>[2x]MKRVITLFAVLLMGWSVNAWSFACKTANGTAIPIGGGSANVYVNLAPVVNVGQNLVVDLSTQIFCHNDYPETITDYVTLQRGSAYGGVLSNFSGTVKYSGSSYPFPTTSETPRVVYNSRTDKPWPVALYLTPVSSAGGVAIKAGSLIAVLILRQTNNYNSDDFQFVWNIYANNDVVVPTGGCDVSARDVTVTLPDYPGSVPIPLTVYCAKSQNLGYYLSGTTADAGNSIFTNTASFSPAQGVG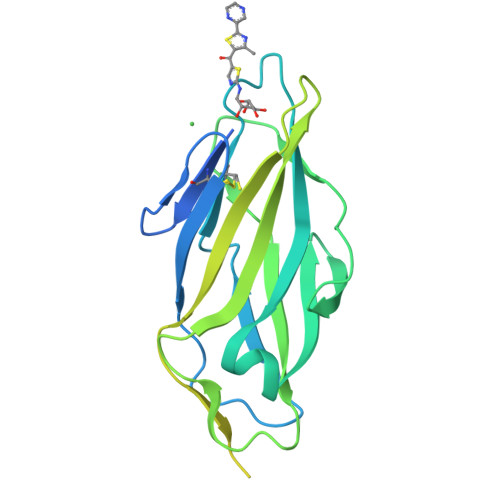VQLTRNGTIIPANNTVSLGAVGTSAVSLGLTANYARTGGQVTAGNVQSIIGVTFVYQ>[2x]MLLEAIFHEAKGSYAYPISETQLRVRLRAKKGDVVRCEVLYADRYASPEEELAHALAGKAGSDERFDYFEALLECSTKRVKYVFLLTGPQGEAVYFGETGFSAERSKAGVFQYAYIHRSEVFTTPEWAKEAVIYQIFPERFANGDPSNDPPGTEQWAKDARPRHDSFYGGDLKGVIDRLPYLEELGVTALYFTPIFASPSHHKYDTADYLAIDPQFGDLPTFRRLVDEAHRRGIKIILDAVFNHAGDQFFAFRDVLQKGEQSRYKDWFFIEDFPVSKTSRTNYETFAVQVPAMPKLRTENPEVKEYLFDVARFWMEQGIDGWRLDVANEVDHAFWREFRRLVKSLNPDALIVGEIWHDASGWLMGDQFDSVMNYLFRESVIRFFATGEIHAERFDAELTRARMLYPEQAAQGLWNLLDSHDTERFLTSCGGNEAKFRLAVLFQMTYLGTP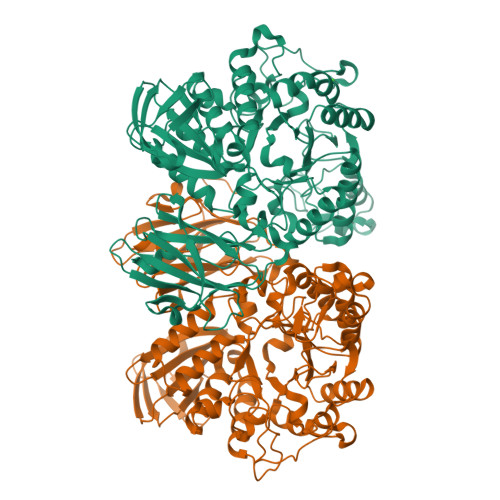LIYYGDEIGMAGATDPDCLRPMIWEEKEQNRGLFEFYKELIRLRHRLASLTRGNVRSWHADKQANLYAFVRTVQDQHVGVVLNNRGEKQTVLLQVPESGGKTWLDCLTGEEVHGKQGQLKLTLRPYQGMILWNGR> SMDEADRRLLRRCRLRLVEELQVDQLWDVLLSRELFRPHMIEDIQRAGSGSRRDQARQLIIDLETRGSQALPLFISCLEDTG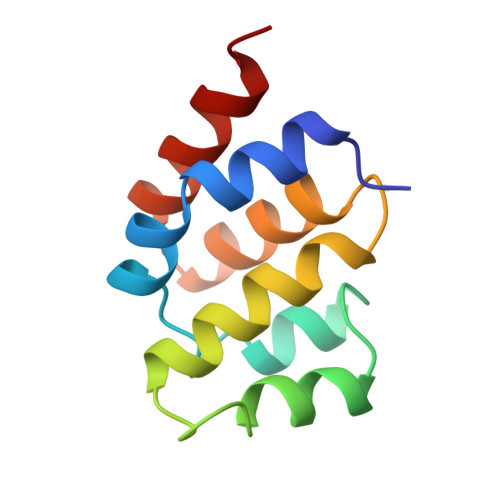QDMLASFLRTNRQAG> CEKACNPRMGNLALGRKLRADTMCGQNATELFCFYSENADLTCRQPKCDKCNAAHSHLAHPPSAMADSSFRFPRTWW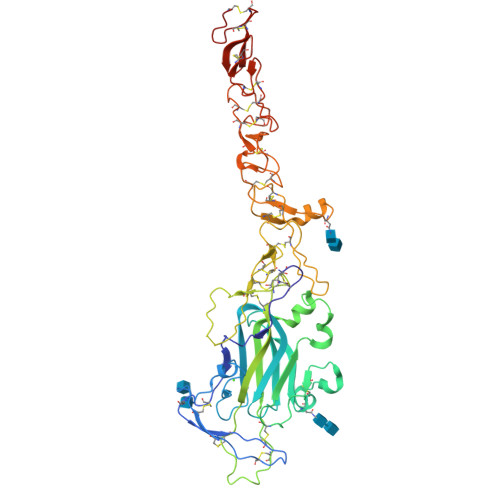QSAEDVHREKIQLDLEAEFYFTHLIMVFKSPRPAAMVLDRSQDFGKTWKPYKYFATNCSATFGLEDDVVKKGAICTSRYSNPFPCTGGEVIFRALSPPYDIENPYSAKVQEQLKITNLRVRLLKRQSCPCQINDLNAKPHHFMHYAVYDFIVKGSCFCNGHADQCLPVEGFRPIKAPGAFHVVHGRCMCKHNTAGSHCQHCAPLYNDRPWEAADGRTGAPNECRTCKCNGHADTCHFDVNVWEASGNRSGGVCNNCQHNTEGQHCQRCKPGFYRDLRRPFSAPDACKACSCHPVGSAILPFSSVTFCDPSNGDCPCKPGVAGPHCDRCMVGYWGFGDYGCRPCDCAGSCDPLTGDC> GSDNIISFDHVTFTYPDSPRPALSDLSFAIERGSWTALIGHNGSGKSTVSKLINGLLAPDDLDKSSITVDGVKLGADTVWEVREKVGIVFQNPDNQFVGATVSDDVAFGLENRAVPRPEMLKIVAQAVADVGMADYADSEPSNLSGGQKQRVAIAGILAVKPQVIILDESTSMLDPEGKEQI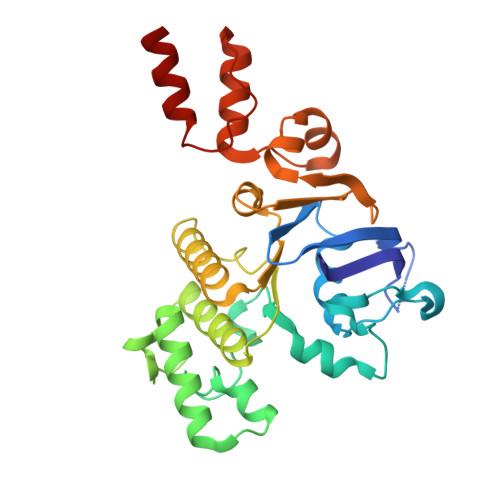LDLVRKIKEDNNLTVISITHDLEEAAGADQVLVLDDGQLLDQGKPEEIFPKVEMLKRIGLDIPFVYRLKQLLKERGIVLPDEIDDDEKLVQSLWQLNSKM> SVPIVSAWEKGMEA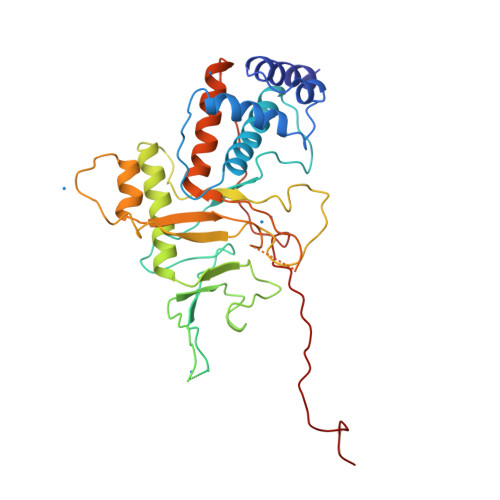ARALMDKYHVDNDLKANFKLLPDQVEALAAVCKTWLNEEHRGLQLTFTSNKTFVTMMGRFLQAYLQSFAEVTYKHHEPTGCALWLHRCAEIEGELKCLHGSIMINKEHVIEMDVTSENGQRALKEQSSKAKIVKNRWGRNVVQISNTDARCCVHDAACPANQFSGKSCGMFFSEGAKAQVAFKQIKAFMQALYPNAQTGHGHLLMPLRCECNSKPGHAPFLGRQLPKLTPFALSNAEDLDADLISDKSVLASVHHPALIVFQCCNPVYRNSRAQGGGPNCDFKISAPDLLNALVMVRSLWSENFTELPRMVVPEFKWSTKHQYRNVSLPVAHSDARQNPFDF>[2x]MGCGGTADKNPAGNNGDSAKPAETKSGDSVSLTLRHINVRDTAKNTLALLEKVVKKTEAEVPGATFKLDGVEDTVNRDVKLKAEMAAGKPPQIFNLFGGADTQNYAKAGHLLPLNDILKELGLEDKFFELREFTVDGKIYGLPEAGFVEGFYYNTKLFADAGITSAPKTWDEFTKA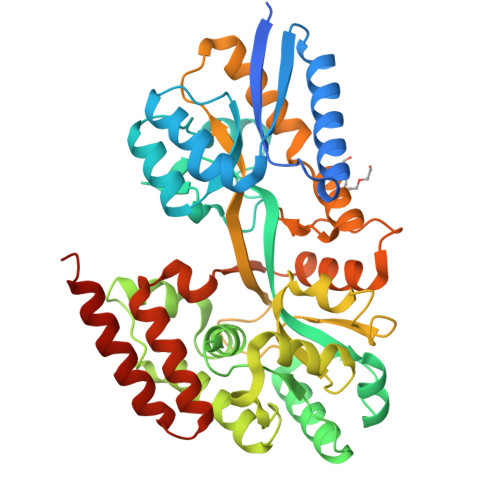LEALKAKNITPIALGGGSGDGWAINMLANSLFVATAGPEAQEGFAKGTTKWTDPAVLDGFKRLKDLKDKGYIDPNVLGLKYSEGQAKFYTGQAAMLFDGSWATSAILDKDKSTVKDNVGYFRFPNIGGKGDNLINGGWSNGYGFSSHLNDAEKKAVKAFIKNFYTLEIQGEALGRDNRVPSMKGVPTPAEAAPLTKAIGEAQASAKAAFPAFDALVQPKVKVTLEQSVQELLGGQLTPEKLVEKMQKVQDEANAGKLEHHHHHH>SRSTHNEMEKNRRAHLRLSLEKLKGLVPLGPDSSRHTTLSLLTKAKLHIKKLEDSDRKAVHQIDQLQREQRHLKRQLEKL[2x];>KRAHHNALERKRRDHIKDSFHSLRDSVPSLQGEKASRAQILDKATEYIQYMRRKNH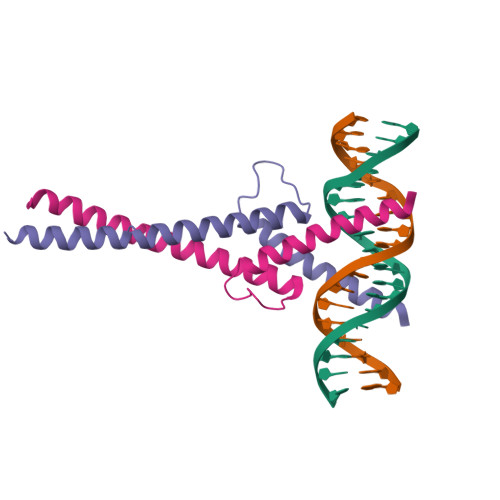THQQDIDDLKRQNALLEQQV[2x]> HPETLVKVKDAEDQLGARVGYIELDLNSGKILESFRPEERFPMMSTFKVLLCGAVLSRVDAGQEQLGRRIHYSQNDLVEYSPVTEKHLTDGMTVRELCSAAITM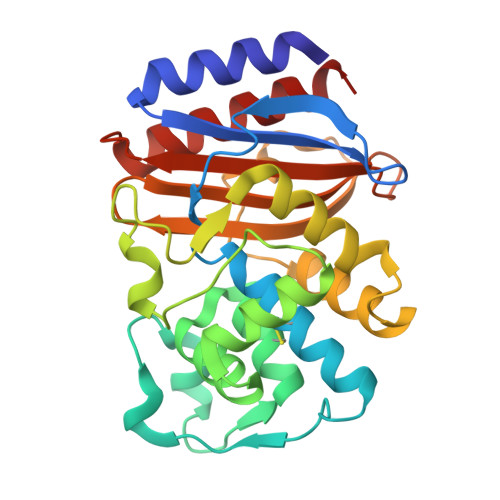SDNTAANLLLTTIGGPKELTAFLHNMGDHVTRLDRWEPELNEAIPNDERDTTMPAAMATTLRKLLTGELLTLASRQQLIDWMEADKVAGPLLRSALPAGWFIADKSGAGERGSRGIIAALGPDGKPSRIVVIYTTGSQATMDERNRQIAEIGASLIKHW> HAYIVKSSPGENSELKSAPAQVEIEFNEPVEEGFHYIKVYNSNGDRVDTDKTEIKKDNHHIMTVKLKKNLPKDVYRAEWNAVSADGHPVSGVIPFSI

The ycnKJI operon in B. subtilis encodes a suite of proteins implicated in Cu uptake and regulation, including the Cu-binding protein YcnI and the putative Cu importer YcnJ. The YcnJ protein has two extracellular domains (an N-terminal CopC domain and a C-terminal YtkA domain), which sandwich a membrane-embedded CopD domain. YcnJ from B. subtilis has been implicated as a Cu importer, proposed to use its membrane-bound CopD domain for Cu uptake. Here, we demonstrate that one of the extracellular domains within YcnJ (YcnJCopC) binds Cu(II) in 1:1 stoichiometry with high affinity using a histidine brace motif.

We purified the resulting YcnJCopC protein and crystallized it in its as-purified, apo form. We determined its structure to 0.160 nm (1.60 Å) resolution. The overall fold displays the typical β-barrel structure of a cupredoxin fold observed in other CopC proteins. Of those CopC homologs whose structures have been experimentally determined, YcnJCopC has the lowest RMSD with the Cu(II)-binding CopC protein from Methylosinus trichosporium OB3b. The main difference between YcnJCopC and these other proteins is a disruption of β4. This could, however, be a crystallization artifact, since we also observe electron density for triethylene glycol and a sulfate ion from the crystallization solution near this beta strand. Another His and an Asp from a DxH motif provide a third coordinating nitrogen and a coordinating oxygen, respectively. These three residues are conserved in YcnJCopC, and the crystal structure shows that these amino acids are close to one another, suggesting that they may be involved in Cu binding similar to other metalated proteins in this family. On the other hand, in its apo form, YcnJCopC has π–π stacking between the two imidazole rings of the two conserved His side chains, an interaction not accessible to YcnI because it lacks a second His ligand. Concurrently, in the absence of Cu, the two His ligands in YcnJCopC can engage in π–π stacking, as we observe in our crystal structure. Protonation of histidines also helps to stabilize these π–π interactions, so Cu binding may also destabilize π–π stacking.>QKQLRGQIARRVYRQLLAEKRAEEEKRKREEEEKRKREEEERERERERREAELRAQQEEAARKQRELEALQQESQRAAELSRELEKQKENKQVEEILRLEKEIEDLQRMKERQELSLTEASLQKLQQLRDEELR[2x]

Class X myosin has been found to be localized at the tips of filopodia, which are plasma membrane protrusions containing bundled actin that are necessary for cellular processes such as cell adhesion, migration, angiogenesis and the formation of cell–cell contacts. Myosin X is required for filopodia formation and extension. Myosin motors move along actin filaments via a series of conformational changes in the motor domain that are coupled with the sequential release of MgATP hydrolysis products, Pi and MgADP. These conformational changes in the motor domain are amplified by the myosin lever arm, which is comprized of the C-terminal subdomain of the motor domain (known as the converter) and an extended alpha helix length that varies with the myosin class12.

We have obtained crystals of this critical region that contain the IQ3, SAH and dimerization region (L786-A932). From the resulting structure at 3.5 Å resolution, it is clear that the SAH (E814-A846) and the following helical region (E847-E884) together form a 10.5 nm long single α-helix and elongates the IQ region. The structure also reveals how the two SAH regions are joined together by an anti-parallel coiled-coil. The boundary between the SAH and the region that participates in the anti-parallel coiled-coil is not evident from the sequence, but is evident in the new structure, and results in an SAH that is shorter than suggested for a monomeric construct14. The anti-parallel coiled-coil that is formed is in agreement with the NMR structure. The structure and dynamics of the SAH-CC-SAH dimeric region is particularly important to allow inferences as to the lever arm rigidity, which will dictate the space that a lead head can explore while the rear head is attached to actin. Molecular dynamic simulations of this region show that no melting of the SAH occurs on the simulation timescale, although bending (or twisting) is possible within the SAH. Interestingly, the simulation promotes a spontaneous relaxation of the SAH-CC-SAH structure that stretches this region by 1.7 nm relative to the X-ray structure, reaching a value of 25.7 nm. The structure of the ‘hinge' of the motor that connects the two heads of a dimer is thus described for the first time, as well as the length and structure of the lever arm and the dimerization region of myosin X in its native context.> HHHHHHSSGLVPRGSHMASMLDMDDLATL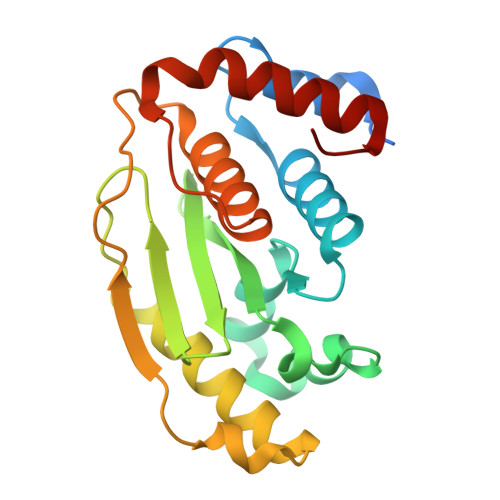DGQNWLNDQVINMYGELIMDAVPDKVHFFNSFFHRQLVTKGYNGVKRWTKKVDLFKKSLLLIPIHLEVHWSLITVTLSNRIISFYDSQGIHFKFCVENIRKYLLTEAREKNRPEFLQGWQTAVTKCIPQQKNDSDCGVFVLQYCKCLALEQPFQFSQEDMPRVRKRIYKELCECRLMD>[2x]GFKQDIATIRGDLRTYAQDIFLAFLNKYPDERRYFKNYVGKSDQELKSMAKFGDHTEKV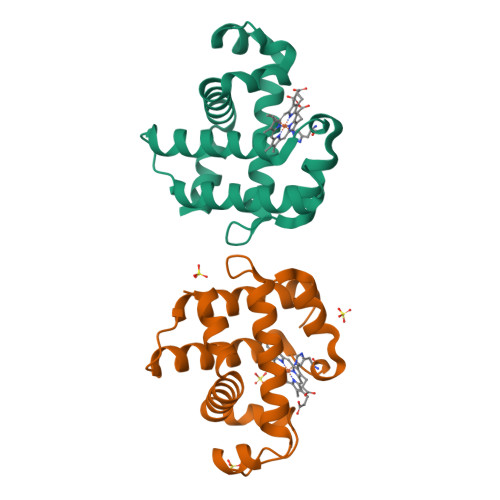FNLMMEVADRATDCVPLASDANTLVQMKQHSSLTTGNFEKLFVALVEYMRASGQSFDSQSWDRFGKNLVSALSSAGMK> KKNIKRNVEKIIAQWDERTRKNKENFDFGELTLSTGLPGIILMLAELKNKDNSKIYQKKIDNYIEYIVSKLSTYGLLTGSLYSGAAGIALSILHLREDDEKYKNLLDSLNRYIEYFVREKIEGFNLENITPPDYDVIEGLSGILSYLLLINDEQYDDLKILIINFLSNLTKENNGLISLYIKSENQMSQSESEMYPLGCLNMGLAHGLAGV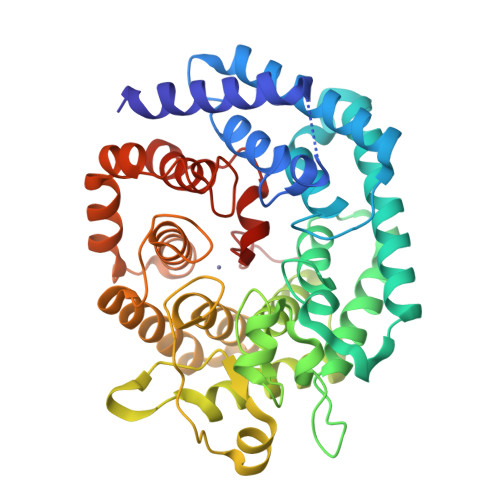GCILAYAHIKGYSNEASLSALQKIIFIYEKFELERKKQFLWKDGLVADELKKEKVIREASFIRDAWCYGGPGISLLYLYGGLALDNDYFVDKAEKILESAMQRKLGIDSYMICHGYSGLIEICSLFKRLLNTKKFDSYMEEFNVNSEQILEEYGDESGTGFLEGISGCILVLSKFEYSINFTYWRQALLLFDDFLKGG> MANELTWHDVLAEEKQQPYFLNTLQTVASERQSGVTIYPPQKDVFNAFRFTELGDVKVVILGQDPYHGPGQAHGLAFSVRPGIAIPPSLLNMYKELENTIPGFTRPNHGYLESWARQGVLLLNTVLTVRAGQAHSHASLGWETFTDKVISLINQHREGVVFLLWGSHAQKKGAIIDKQRHHVLKAPDPSPLSAHRGFFGCNHFVLANQWLEQRGETPI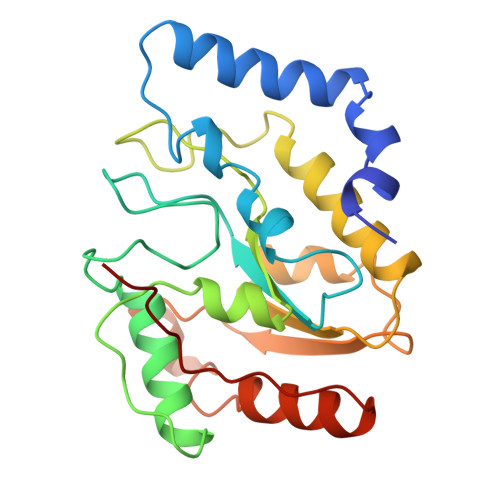DWMPVLPAESE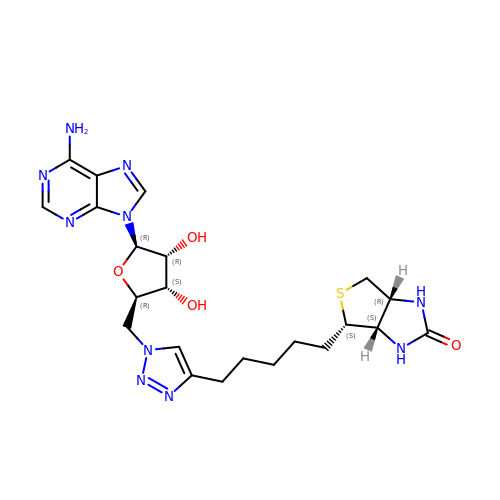5'-deoxy-5'-(4-{5-[(3aS,4S,6aR)-2-oxohexahydro-1H-thieno[3,4-d]imidazol-4-yl]pentyl}-1H-1,2,3-triazol-1-yl)adenosine | C22 H30 N10 O4 S | PNZFOGQAKKAJAB-ZOFBHSOPSA-N>MAPFPEEVDVFTAPHWRMKQLVGLYCDKLSKTNFSNNNDFRALLQSLYATFKEFKMHEQIENEYIIGLLQQRSQTIYNVHSDNKLSEMLSLFEKGLKNVKNEYEQLNYAKQLKERLEAFTRDFLP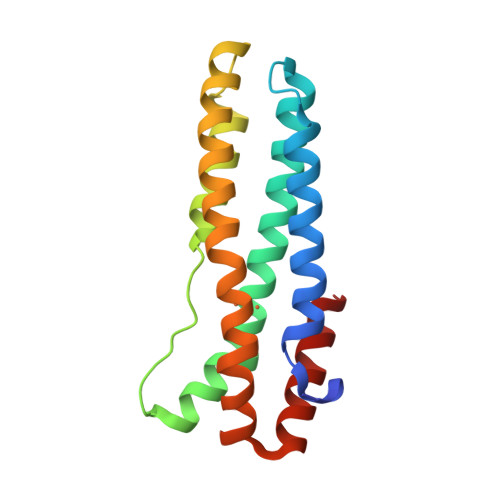HMKEEEEVFQPMLMEYFTYEELKDIKKKVIAQHCS[4x]> SNMWVIGKSKAQDAKAIMVNGPQFGWYAPAYTYGIGLHGAGYDVTGNTPFAYPGLVFGHNGVISWGSTAGFGDDVDIFAERLSAEKPGYYLHNGKWVKMLSREETITVKNGQAETFTVWRTVHGNILQTDQTTQTAYAKSRAWDGKELASLLAWTHQMKAKNWQEWTQQAAKQALTINWYYADVNGNIGYVHTGAYPDRQSGHDPRLPVPGTGKWDWKGLLPFEMNPKVYNPQSGYIANWNNSPQKDYPASDLFAFLWGGADRVTEIDRLLEQKPRLTADQAWDVIR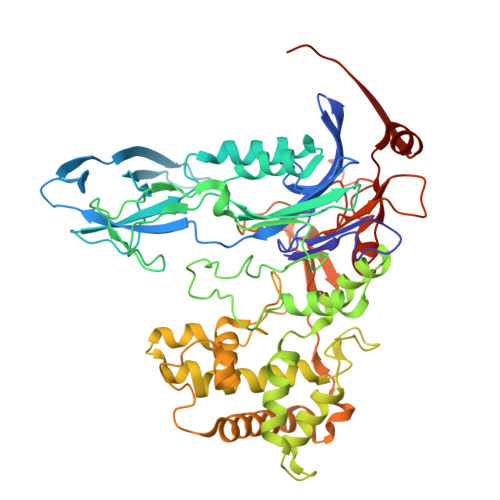QTSRQDLNLRLFLPTLQAATSGLTQSDPRRQLVETLTRWDGINLLNDDGKTWQQPGSAILNVWLTSMLKRTVVAAVPMPFDKWYSASGYETTQDGPTGSLNISVGAKILYEAVQGDKSPIPQAVDLFAGKPQQEVVLAALEDTWETLSKRYGNNVSNWKTPAMALTFRANNFFGVPQAAAEETRHQAEYQNRGTENDMIVFSPTTSDRPVLAWDVVAPGQSGFIAPDGTVDKHYEDQLKMYENFGRKSLWLTKQDVEAHKESQEVLHVQR Terretonin C | C24 H30 O7 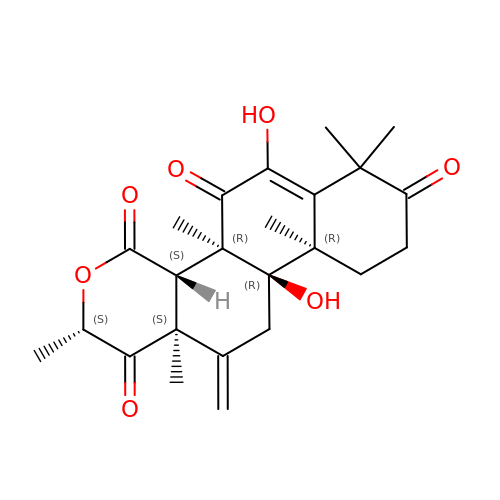| BSUMMOUMVQVPGZ-JUKAANMSSA-N> MSNAALATAPHALELDVHPVAGRIGAEIRGVKLSPDLDAATVEAIQAALVRHKVIFFRGQTH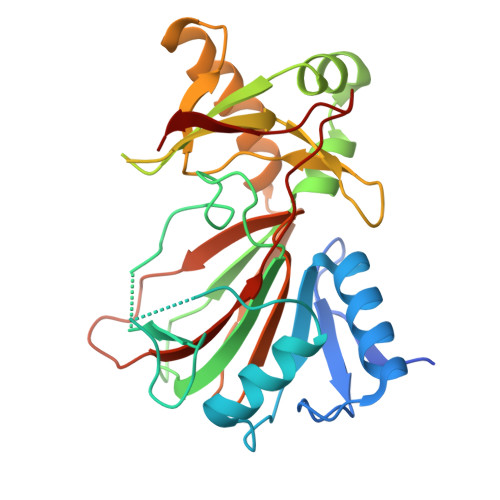LDDQSQEGFAKLLGEPVAHPTVPVVDGTRYLLQLDGAQGQRANSWHTDVTFVEAYPKASILRSVVAPASGGDTVWANTAAAYQELPEPLRELADKLWAVHSNRYDYASLKPDIDPAKLERHRKVFTSTVYETEHPVVRVHPISGERALQLGHFVKRIKGYSLADSQHLFAVLQGHVTRLENTVRWRWEAGDVAIWDNRATQHYAVDDYGTQPRIVRRVTLAGEVPVGVDGQLSRTTRKG>[2x]SVLFPCKYASSGCEITLPHTEKAEHEELCEFRPYSCPCPGASCKWQGSLDAVMPHLMHQHKSITTLQGEDIVFLATDINLPGAVDWVMMQSCFGFHF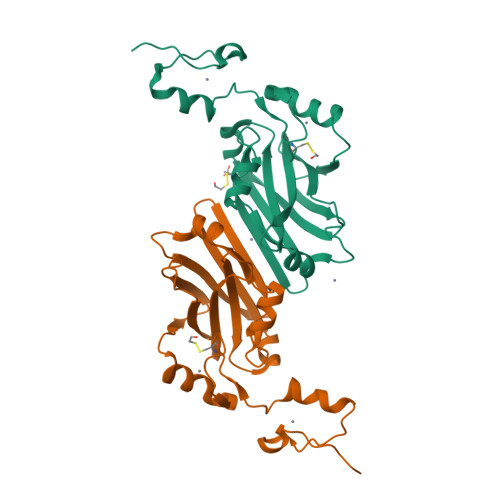MLVLEKQEKYDGHQQFFAIVQLIGTRKQAENFAYRLELNGHRRRLTWEATPRSIHEGIATAIMNSDCLVFDTSIAQLFAENGNLGINVTISMC>MEPEAPRRRHTHQRGYLLTRNPHLNKDLAFTLEERQQLNIHGLLPPSFNSQEIQVLRVVKNFEHLNSDFDRYLLLMDLQDRNEKLFYRVLTSDIEKFMPIVYTPTVGLACQQYSLVFRKPRGLFITIHDRGHIASVLNAWPEDVIKAIVVTDGERILGLGDLGCNGMGIPVGKLALYTACGGMNPQECLPVILDVGTENEELLKDPLYIGLRQRRVRGSEYDDFLDEFMEAVSSKYGMNCLIQFEDFANVNAFRLLNKYRNQYCTFNDDIQGTASVAVAGLLAALRITKNKLSDQTILFQGAGEAALGIAHLIVMALEKEGLPKEKAIKKIWLVDSKGLIVKGRASLTQEKEKFAHEHEEMKNLEAIVQEIKPTALIGVAAIGGAFSEQILKDMAAFNERPIIFALSNPTSKAECSAEQCYKITKGRAIFASGSPFDPVTLPNGQTLYPGQGNNSYVFPGVALGVVACGLRQITDNIFLTTAEVIAQQVSDKHLEEGRLYPPLNTIRDVSLKIAEKIVKDAYQEKTATVYPEPQNKEAFVR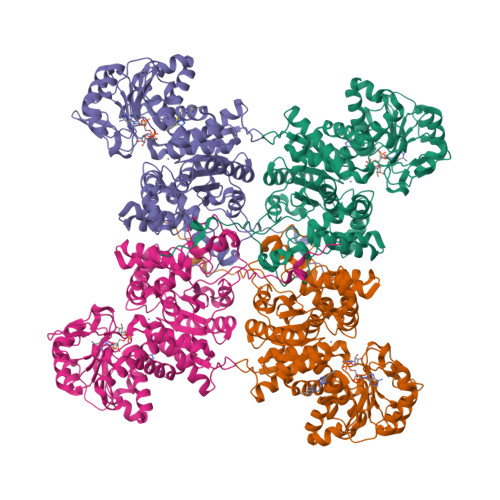SQMYSTDYDQILPDCYSWPEEVQKIQTKVDQ[4x]>GSHMKDYSLEIDAVMKAAQINDTNNFVQALMRWHFSKETGSPFWLGMREQLNFDPIKDVKTINDLRQFSDISHCLRQEPVANLVPQGLPADSHPQVYESGGTTGAPKYVVAYDAWIEALISWRMSGYQHRPGRPSGNTLAAIPTGPHIVGAINKERALRLGGMFFSIDIDPRWVKRSLSEGDTATVRKYTHHLVDQVQNTLMNQDIRFLVTTPPVLRELLKRPEVVLQMKQSLAQITLGGTELNLDEIKFIASEILPDCEFSASYGSTSALGVSRSLLITSESQQVIYDSFSPFITYDVVDSITAQTVEYGERGNVIVTHLSPWAFYPRVAERDTAIRLPGVSGFAG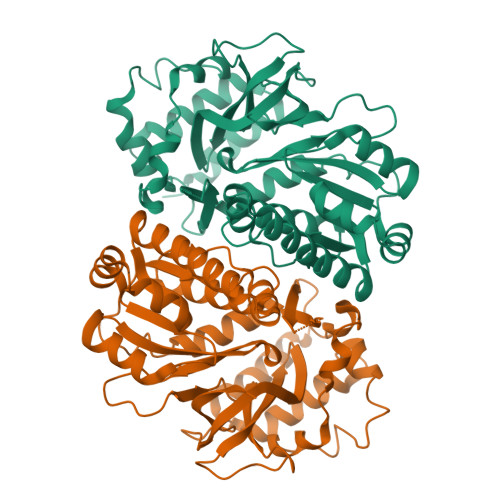DRLADIEPLKISEGRKVIEGVY[2x]> SMLKREDWYDLTRTTNWTPKYVTENELFPEEMSGARGISMEAWEKYDEPYKITYPEYVSIQREKDSGAYSIKAA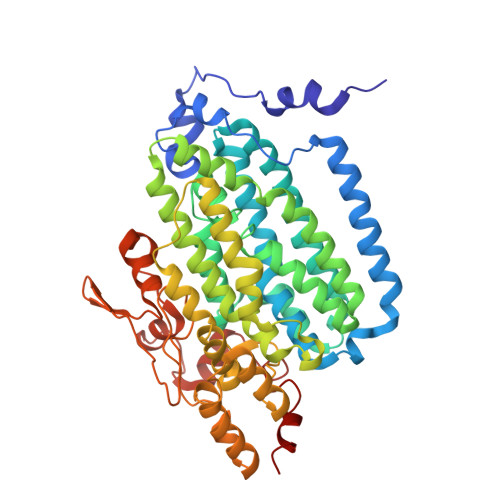LERDGFVDRADPGWVSTMQLHFGAIALEEYAASTAEARMARFAKAPGNRNMATFGMMDENRHGQIQLYFPYANVKRSRKWDWAHKAIHTNEWAAIAARSFFDDMMMTRDSVAVSIMLTFAFETGFTNMQFLGLAADAAEAGDHTFASLISSIQTDESRHAQQGGPSLKILVENGKKDEAQQMVDVAIWRSWKLFSVLTGPIMDYYTPLESRNQSFKEFMLEWIVAQFERQLLDLGLDKPWYWDQFMQDLDETHHGMHLGVWYWRPTVWWDPAAGVSPEEREWLEEKYPGWNDTWGQCWDVITDNLVNGKPELTVPETLPTICNMCNLPIAHTPGNKWNVKDYQLEYEGRLYHFGSEADRWCFQIDPERYKNHTNLVDRFLKGEIQPADLAGALMYMSLEPGVMGDDAHDYEWVKAYQ>GSPEFPGMSQSNRELVVDFLSYKLSQKGYSWSQFSDVEENRTEAPEETEPERETPSAINGNPSWHLADSPAVNGATGHSSSLDAREVIPMAAVKQALREAGDEFELRYRRAFSDLTSQLHITPGTAYQSFEQVVNELFRDG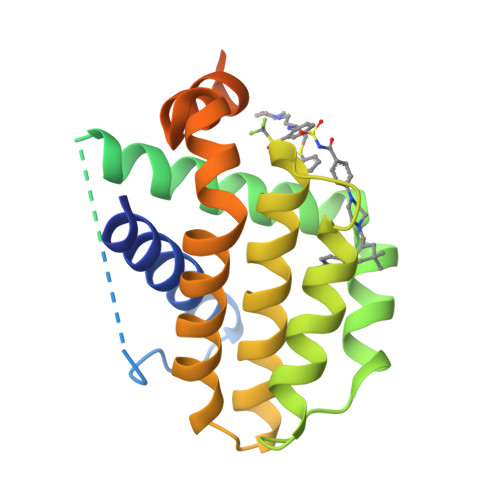VNWGRIVAFFSFGGALCVESVDKEMQVLVSRIASWMATYLNDHLEPWIQENGGWDTFVDLYGNNAAAESRKGQERFNRWFLTGMTVAGVVLLGSLFSRK[12x]>MQQKLENIKFVITDVDGVLTDGQLHYDANGEAIKSFHVRDGLGIKMLMDADIQVAVLSGRDSPILRRRIADLGIKLFFLGKLEKETACFDLMKQAGVTAEQTAYIGDDSVDLPAFA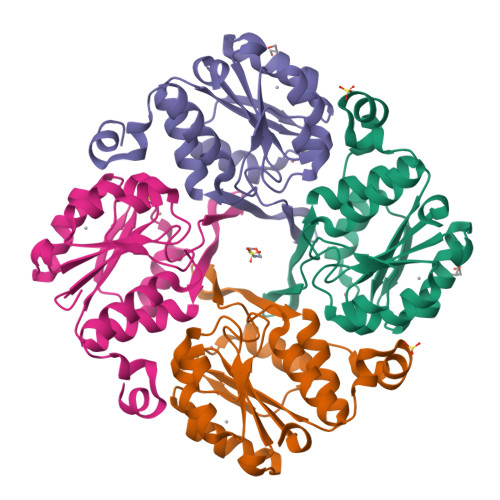ACGTSFAVADAPIYVKNAVDHVLSTHGGKGAFREMSDMILQAQGKSSVFDTAQGFLKSVKSMGQ[12x]> LGKTR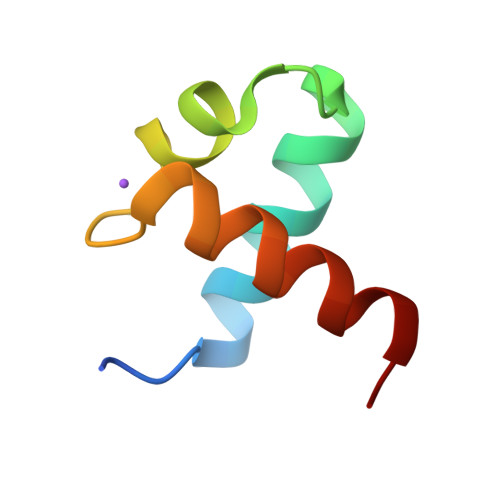WTREEDEKLKKLVEQNGTDDWKVIANYLPNRTDVQCQHRWQKVLNPE>[2x]MDFNLTDIQQDFLKLAHDFGEKKLAPTVTERDHKGIYDKELIDELLSLGITGAYFEEKYGGSGDDGGDVLSYILAVEELAKYDAGVAITLSATVSLCANPIWQFGTEAQKEKFLVPLV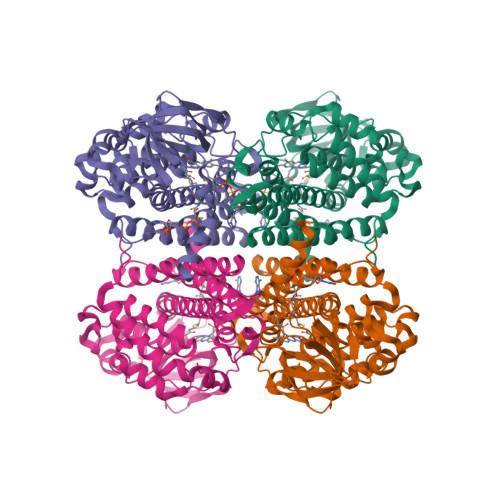EGTKLGAFGLTEPNAGTDASGQQTIATKNDDGTYTLNGSKIFITNGGAADIYIVFAMTDKSKGNHGITAFILEDGTPGFTYGKKEDKMGIHTSQTMELVFQDVKVPAENMLGEEGKGFKIAMMTLDGGRIGVAAQALGIAEAALADAVEYSKQRVQFGKPLCKFQSISFKLADMKMQIEAARNLVYKAACKKQEGKPFTVDAAIAKRVASDVAMRVTTEAVQIFGGYGYSEEYPVARHMRDAKITQIYEGTNEVQLMVTGGALLR>[4x]MRGSHHHHHHGSSQVADKDDPTNKFYQSVIQLGNGFLDVFTSFGGLVAEAFGFKSD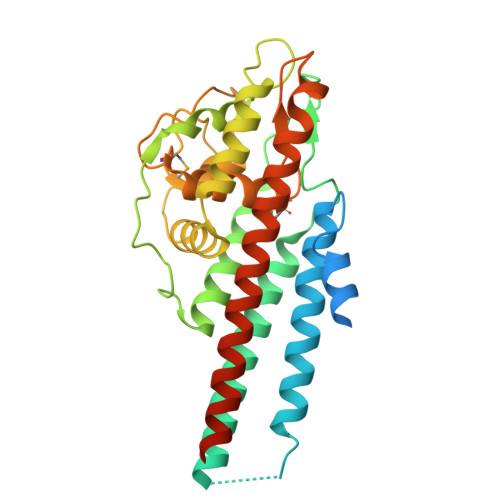PKKSDVKTYFTTVAAKLEKTKTDLNSLPKEKSDISSTTGKPDSTGSVGTAVEGAIKEVSELLDKLVKAVKTAEGASSGTAAIGEVVADADAAKVADKASVKGIAKGIKEIVEAAGGSEKLKAVAAAKGENNKGAGKLFGKAGAAAHGDSEAASKAAGAVSAVSGEQILSAIVTAADAAEQDGKKPEEAKNPIAAAIGDKDGGAEFGQDEMKKDDQIAAAIALRGMAKDGKFAVKDGEKEKAEGAIKGAAESAVRKVLGAITGLIGDAVSSGLRKVGDSVKAASKETPPALNK> MKDNTVPLKLIALLANGEFHSGEQLGETLGMSRAAINKHIQTLRDWGVDVFTVPGKGYSLPEPIQLLNAKQILGQLDGGSVAVLPVIDSTNQYLLDRIGELKSGDACIAEYQQAGRGRRGRKWFSPFGANLYLSMFWRLEQAPAAAIGLSL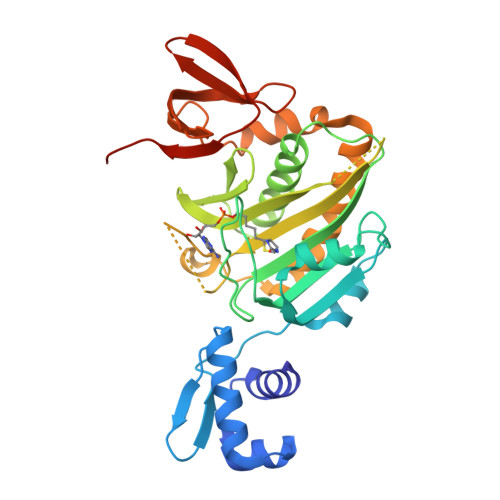VIGIVMAEVLRKLGADKVRVKWPNDLYLQDRKLAGILVELTGKTGDAAQIVIGAGINMAMRRVEESVVNQGWITLQEAGINLDRNTLAAMLIRELRAALELFEQEGLAPYLSRWEKLDNFINRPVKLIIGDKEIFGISRGIDKQGALLLEQDGIIKPWMGGEISLRSAEKHHHHHH>[2x]SNRLDGKVAIITGGTLGIGLAIATKFVEEGAKVMITGRHSDVGEKAAKSVGTPDQIQFFQHDSSDEDGWTKLFDATEKAFGPVSTLVNNAGIAVNKSVEETTTAEWRKLLAVNLDGVFFGTRLGIQRMKNKGLGASIINMSSIEGFVGDPSLGAYNASKGAVRIMSKSAALDCALKDYDVRVNTVHPGYIKTPLVDDLPGAEEAMSQRTKTPMGHIGEP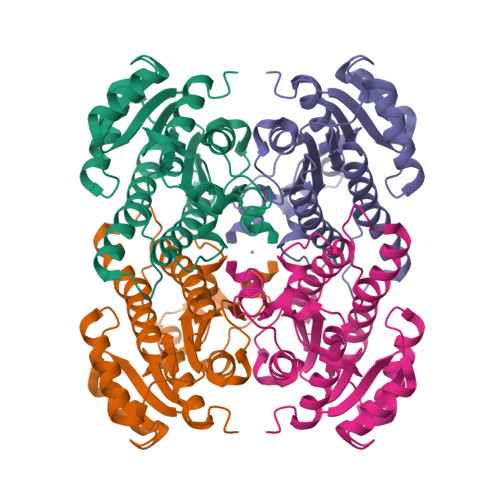NDIAYICVYLASNESKFATGSEFVVDGGYTAQ>GSPEFMELEIRPLFLVPDTNGFIDHLASLARLLESRKYILVVPLIVINELDGLAKGQETDHRAGGYARVVQEKARKSIEFLEQRFESRDSCLRALTSRGNELESIAFRSEDITGQLGNNDDLILSCCLHYCKDKAKDFMPASKEEPIRLLREVVLLTDDRNLRVKALTRNVPVRDI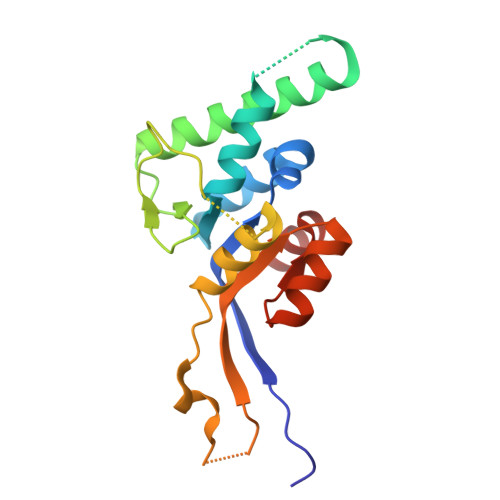PAFLTWAQVG[2x]>[2x]SNALQGKRILITAGPTREKIDPVRFMTNFSSGKMGYAIAEVAVNLGAEVILVSGPTALNPPLHVTTV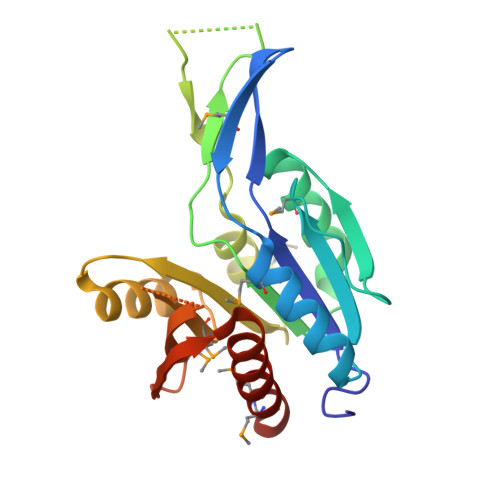QVESAQDMLEAVIQHYQNVDVVIKTAAVADYRPKYVHDNKMKKKNGDAVIELERTVDILKTLGEMKDKQLLIGFAAETTNVEEYATKKLREKNANMIVANDVKAQGAGFGTDTNIVTMYRKDGEVIELPLLTKKEVAREILKQIEMMLEDDRL4-(2-bromoethyl)benzoic acid | C9 H9 Br O2 | 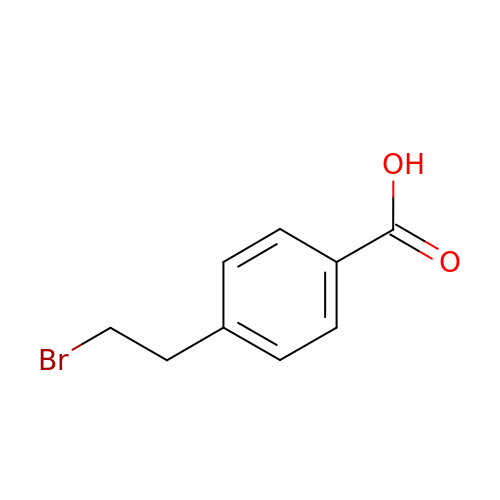BKMRWJWLBHHGCF-UHFFFAOYSA-N>[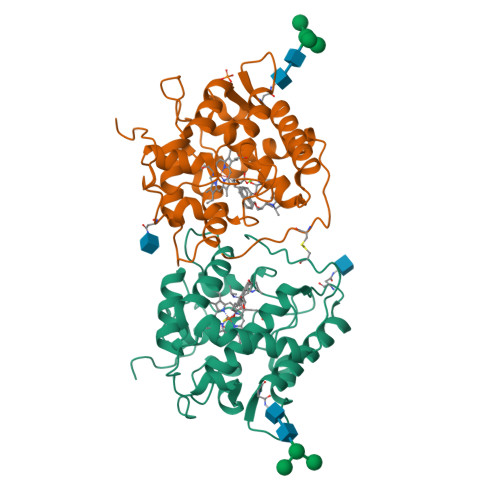2x]SAHPWKAPGPNDSRGPCPGLNTLANHGFLPRNGRNISVPMIVKAGFEGYNVQSDILILAGKIGMLTSREADTISLEDLKLHGTIEHDASLSREDVAIGDNLHFNEAIFTTLANSNPGADVYNISSAAQVQHDRLADSLARNPNVTNTDLTATIRSSESAFFLTVMSAGDPLRGEAPKKFVNVFFREERMPIKEGWKRSTTPITIPLLGPIIERITELSDWKPTGDNCGAIVLSP>APLADYKDDDDKLASTLDYLTGILITRHSQSETVPACSAGHTELWTGYSLLYVDGNDYAHNQDLGSPGSCVPRFSTLPVLSCGQNNVCNYASRNDKTFWLTTNAAIPMMPVENIEIRQYISRCVVCEAPANVIAVHSQTIEVPDCPNGWEGLWIGYSFLMHTAVGNGGGGQALQSPGSCLEDFRATPFIECNGAKGTCHFYETMTSFWMYNLESSQPFERPQQQTIKAGERQSHVSRCQVCMKNSSGSSASSGAPKSRGFIFARHSQSVHVPQCPANTNLLWEGYSLSGNVAASRAVGQDLGQSGSCMMRFTTMPYMLCDITNVCHFAQNNDDSLWLSTAEPMPMTMTPIQGRDLMKYISRCVVCETTTRIIALHSQSMSIPDCPGGWEEMWTGYSYFMSTLDNVGGVGQNLVSPGSCLEEFRAQPVIECHGHGRCNYYDALASFWLTVIEEQDQFVQPRQQTLKADFTSKISRCTVCRRRGNGSSASSGLDYLTGILITRHSQSETVPACSAGHTELWTGYSLLYVDGNDYAHNQDLGSPGSCVPRFSTLPVLSCGQNNVCNYASRNDKTFWLTTNAAIPMMPVENIEIRQYISRCVVCEAPANVIAVHSQTIEVPDCPNGWEGLWIGYSFLMHTAVGNGGGGQALQSPGSCLEDFRATPFIECNGAKGTCHFYETMTSFWMYNLESSQPFERPQQQTIKAGERQSHVSRCQVCMKNSSGSGSGS[2x]

Collagen IV is an essential structural protein in all metazoans. It provides a scaffold for the assembly of basement membranes, a specialized form of extracellular matrix, which anchors and signals cells and provides microscale tensile strength. Scaffolds are composed of α-chains that coassemble into triple-helical protomers of distinct chain compositions, which in turn oligomerize into supramolecular scaffolds. We solved the crystal structure of the NC1 hexamer, determined the chain composition of protomers, and found that Drosophila adapted an evolutionarily unique mechanism of scaffold assembly that requires divalent cations.

To overcome this problem, we recombinantly produced FLAG-tagged single-chain NC1 trimers with specific hetero-compositions CVC and VCV using the same design as in transgenic analysis but without a fluorescent protein. Thus, the CVC composition of NC1 was able to spontaneously form a hexamer although this process was highly inefficient. Moreover, once assembled the CVC hexamer was not dependent on chloride pressure, thus confirming the Cl- independent mechanism of stability. We were able to obtain diffracting crystals of tissue-extracted NC1 hexamer (at 2.98 Å resolution) and CVC trimer (at 1.75 Å resolution) and solved their atomic structures. We solved the crystal structures of tissue-extracted and recombinant NC1 hexamers and found that the tissue-extracted complex is indeed a heterotrimer of the same composition as the recombinant CVC single-chain construct. RMSD of superimposed recombinant and tissue-extracted structures of Drosophila NC1 hexamer is 0.43 Å between 1346 pruned atom pairs (across all 1351 pairs: 0.47 Å). Analogously to human crystal structures of α112 and α345 NC1 hexamers, we found multiple PEG molecules associated on the surface and in the inner cavity of the Drosophila NC1 hexamer. Instead, two magnesium ions were found at the trimer–trimer interface. Single D40(1590) of Cg25c directly forms a salt bridge with Mg2+, while K79(1629) of the same Cg25c chain and D79(1589) of the Vkg chain interact with water molecules clustered around the divalent cation. Collectively, unlike in mammals Drosophila NC1 hexamer interface is stabilized by four Cl- and two Mg2+ ions.> SPQPLEQIKLSESQLSGRVGMIEMDLASGRTLTAWRADERFPMMCTFKVVLCGAVLARVDAGDEQLERKIHYRQQDLVDYSPVSEKHLADGMTVGELCAAAITMSDNSAA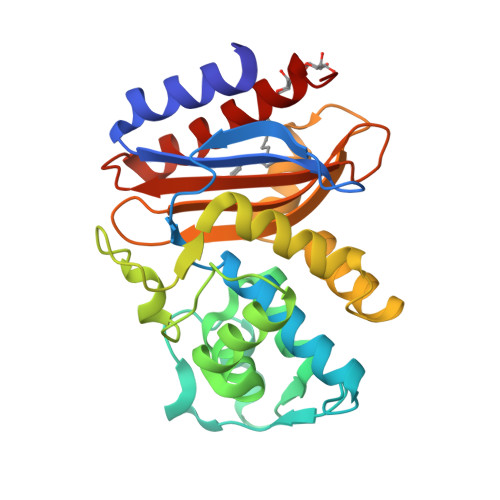NLLLATVGGPAGLTAFLRQIGDNVTRLDRWETELNEALPGDARDTTTPASMAATLRKLLTSQRLSARSQRQLLQWMVDDRVAGPLIRSVLPAGWFIADKTGAGERGARGIVALLGPNNKAERIVVIYLRDTPASMAERNQQIAGIGAALIEHWQR> MNPIHDRTSDYHKYLKVKQGDSDLFKLTVSDKRYIWYNPDPKERDSYECGEIVSETSDSFTFKTVDGQDRQVKKDDANQRNPIKFDGVEDMSELSYLNEPAVFHNLRVRYNQDLIYTYSGLFLVAVNPFKRIPIYTQEMVDIFKGRRRNEVAPHIFAISDVAYRSMLDDRQNQSLLITGESGAGKTENTKKVIQYLASVAGRNQANGSGVLEQQILQANPILEAFGNAKTTRNNNSSRFGKFIEIQFNSAGFISGASIQSYLLEKSRVVFQSETERNYHIFYQLLAGATAEEKKALHLAGPESFNYLNQSGCVDI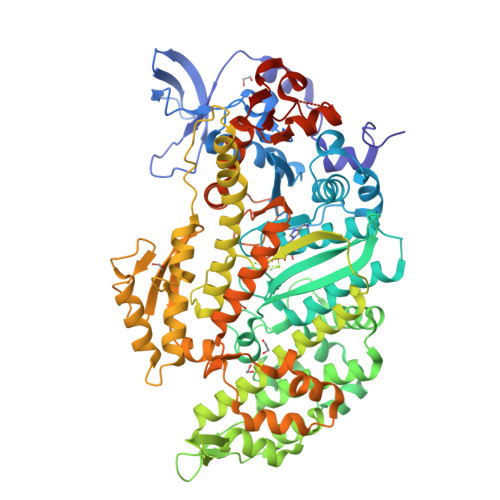KGVSDSEEFKITRQAMDIVGFSQEEQMSIFKIIAGILHLGNIKFEKGAGEGAVLKDKTALNAASTVFGVNPSVLEKALMEPRILAGRDLVAQHLNVEKSSSSRDALVKALYGRLFLWLVKKINNVLCQERKAYFIGVLDIYGFEIFKVNSFEQLCINYTNEKLQQFFNHHMFKLEQEEYLKEKINWTFIDFGLDSQATIDLIDGRQPPGILALLDEQSVFPNATDNTLITKLHSHFSKKNAKYEEPRFSKTEFGVTHYAGQVMYEIQDWLEKNKDPLQQDLELCFKDSSDNVVTKLFNDPNIASRAKKGANFITVAAQYKEQLASLMATLETTNPHFVRCIIPNNKQLPAKLEDKVVLDQLRCNGVLEGIRITRKGFPNRIIYADFVKRYYLLAPNVPRDAEDSQKATDAVLKHLNIDPEQYRFGITKIFFRAGQLARIEEARELRGDYKDDDDK> LKESPSGYLRSGEGDTGCGELVWVGEPLTLRTAETITGKYGVWMRDPKPTYPYTQETTWRIDTVGTDVRQVFEYDLISQFMQGYPSKVHILPRPLESTGAVVYSGSLYFQGAESRTVIRYELNTETVKAEKEIPGAGYHGQFPYSWGGYTDIDLAVDEAGLWVIYSTDEAKGAIVLSKLNPENLELEQTWETNIRKQSVAEAFIICGTLYTVSSYTSADATVNFAYDTGTGISKTLTIPFKNRYKYSSMIKYNPLEKKLFAWDNLNMVTYDIKLSKM

Olfactomedins (OLFs), modular proteins containing an OLF domain that are predominantly expressed in neural tissues, are involved in fundamental processes of cell growth, cell signaling and cell adhesion. High-resolution crystal structures of the ∼30 kDa five-bladed β-propeller OLF domain are available for four subfamily members: olfactomedin-1, latrophilin, myocilin and gliomedin. While the folds are nearly indistinguishable [Fig. 1(a)], one difference is the presence or absence of a heptacoordinate calcium ion bound in the central internal solvent-filled cavity of the β-propeller [Fig. 1(b)]. To survey the OLF triads for calcium binding and to test whether calcium binding can be reverted by simultaneously altering Asn428 to an acidic Asp or Glu, we replaced the triad Asp–Asn–Asp with Asp–Glu–Ser, Asp–Asp–His and Asp–Glu–Lys via site-directed mutagenesis of Asn428 and Asp478.

For myoc-OLFN428E/D478K the difference upon the addition of calcium is within the error of DSF (±2°C), suggesting that myoc-OLFN428E/D478K cannot bind calcium; for myoc-OLFN428D/D478H a marginal stabilization was observed with calcium, suggesting weak if any calcium binding. Instead of not being visible (myoc-OLFD478S), or adopting a well ordered and helical loop at the top face (wild type), residues 260–265 are shifted ∼10 Å from the original top-face helical loop and are now in the approximate location of the myoc-OLFWT side helix. In turn, the residues previously forming the side helix (303–310) form an extended loop conformation. Finally, unlike myoc-OLFD478S, the loop composed of residues 291–295 is ordered, although shifted ∼3 Å from its defined position in myoc-OLFWT. In the central cavity, a salt bridge between Asp380 and Lys478 (2.6 Å) is observed, with the terminal N∊ atom occupying the position of the Na+ ion modeled in myoc-OLFWT. In addition, Lys478 is within hydrogen-bonding distance of the main-chain carbonyls of Gly326 and Leu381, and Asp380 forms a new hydrogen-bonding interaction with Tyr371 (2.7 Å). The position of Tyr371 appears to be shifted ∼0.6 Å compared with the wild type, but still forms a cation–π interaction with Lys423; both of these residues are conserved in Echinodermata OLFs with the Asp–Glu–Lys triad. Like Asn428 in myoc-OLFD478S, Glu428 is no longer in the central cavity and instead forms hydrogen bonds to water molecules present in a cavity between blades D and E. In myoc-OLFWT this cavity is largely hydrophobic, and is lined with Trp373, Val439, Phe467 and Ile477. Overall, OLF domains harboring the Asp–Glu–Lys triad do not appear to be capable of metal-ion binding in the central pore.> GASSAGLGPVVRCEPCDARALAQCAPPPA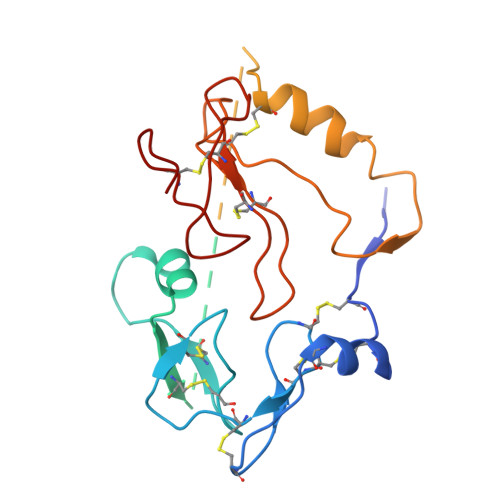VCAELVREPGCGCCLTCALSEGQPCGIYTERCGSGLRCQPSPDEARPLQALLDGRGLCVNASAVSRLRAYLLPAPPAPGNASESEEDRSAGSVESPSVSSTHRVSDPKFHPLHSKIIIIKKGHAKDSQRYKVDYESQSTDTQNFSSESKRETEYGPCRREMEDTLNHLKFLNVLSPRGVHIPNCDKKGFYKKKQCRPSKGRKRGFCWCVDKYGQPLPGYTTKGKEDVHCYSMQSK> GHVETIKNTFLNPKSNKVLVVAHRGNWRSAPENSTAAIDSAIAMKVDIVEIDIQKTKDGQLILMHDNTLDRTTTGKGEIKNWTLADIKKLKLKDKDGKVTNYVVPTLEEALLTAKGKIMVNLDKAYDIFDDVYAILEKTETQNQVIMKGGQPIETVKREFGSYLDKVLYMPVIDLGNKEAEKIITDYL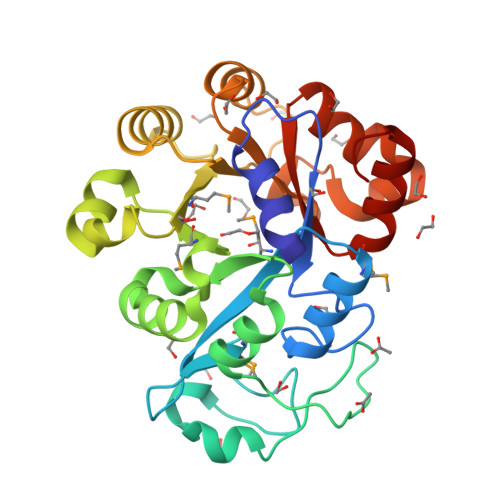KELRPAAFEIIYSDPKNPLPPKIKQLLFKKSLIWYNTLWGSLAGNHDDNLALTDPEKSYGYLIEQLGARILQTDQPAYLLDYLRKKGWHN(2E)-N-hydroxy-3-[1-methyl-4-(phenylacetyl)-1H-pyrrol-2-yl]prop-2-enamide | C16 H16 N2 O3 | 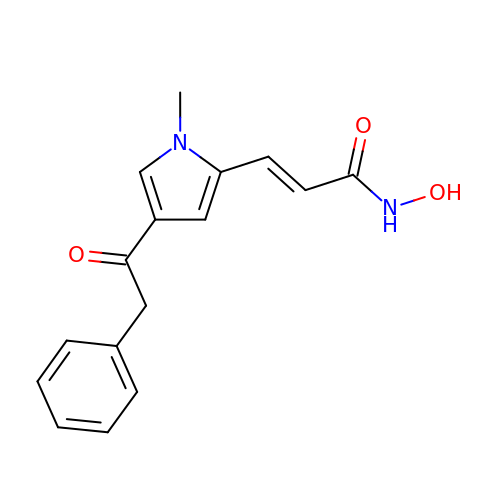UFQOXIMRSMFQRI-BQYQJAHWSA-N>[6x]HHHHHHDYKDDDDKLEVLFQGPEFCKMKKDYRKKYRKYVRSRFQCIEDRNARLGESVSLNKRYTRLRLIKE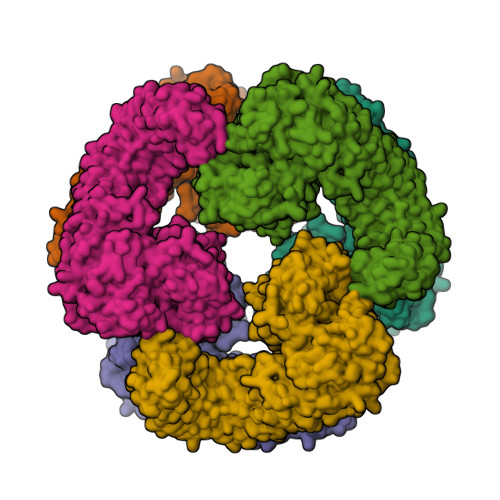HRSQQEREQELLAIGKTKTCESPVSPIKMELLFDPDDEHSEPVHTVVFQGAAGIGKTILARKMMLDWASGTLYQDRFDYLFYIHCREVSLVTQRSLGDLIMSCCPDPNPPIHKIVRKPSRILFLMDGFDELQGAFDEHIGPLCTDWQKAERGDILLSSLIRKKLLPEASLLITTRPVALEKLQHLLDHPRHVEILGFSEAKRKEYFFKYFSDEAQARAAFSLIQENEVLFTMCFIPLVCWIVCTGLKQQMESGKSLAQTSKTTTAVYVFFLSSLLQPRGGSQEHGLCAHLWGLCSLAADGIWNQKILFEESDLRNHGLQKADVSAFLRMNLFQKEVDCEKFYSFIHMTFQEFFAAMYYLLEEEKEGRTNVPGSRLKLPSRDVTVLLENYGKFEKGYLIFVVRFLFGLVNQERTSYLEKKLSCKISQQIRLELLKWIEVKAKAKKLQIQPSQLELFYCLYEMQEEDFVQRAMDYFPKIEINLSTRMDHMVSSFCIENCHRVESLSLGFLHNMPKEEEEEEKEGRHLDMVQCVLPSSSHAACSHGLVNSHLTSSFCRGLFSVLSTSQSLTELDLSDNSLGDPGMRVLCETLQHPGCNIRRLWLGRCGLSHECCFDISLVLSSNQKLVELDLSDNALGDFGIRLLCVGLKHLLCNLKKLWLVSCCLTSACCQDLASVLSTSHSLTRLYVGENALGDSGVAILCEKAKNPQCNLQKLGLVNSGLTSVCCSALSSVLSTNQNLTHLYLRGNTLGDKGIKLLCEGLLHPDCKLQVLELDNCNLTSHCCWDLSTLLTSSQSLRKLSLGNNDLGDLGVMMFCEVLKQQSCLLQNLGLSEMYFNYETKSALETLQEEKPELTVVFEPSW> APLNAARPAEERAALLAWVKERLHEEYGDQDPTPRRDPMHELISTILSQQTTHADEEAAYQELRTLGDWDAITLAPTDAVAHAIRRSNYPESKAPRIQETLRRIKAAPGGYDLDFLRDLPVKDALKWLTDLPGVGVKTASLVLLFNYARPVFPVDTHVHRVSTRVGVIPRMGEQAAHRALLALLPPDPPYLYELHINFLSHGRQVCTWTRPKCGKCILRERCDAYALYGDKVPSFSEKPVKGEKPAKG

Endonuclease III (EndoIII) is a ubiquitous bifunctional DNA glycosylase belonging to the helix-hairpin-helix (HhH)-GDP superfamily of DNA glycosylases. It is active for a broad range of oxidized pyrimidine lesions, removing numerous forms of modified thymine and cytosine bases from DNA, such as thymine glycol (Tg), a major stable oxidative modification of thymine, via the Base Excision Repair (BER) pathway. The crystal structures of EndoIIIs from E. coli (EcEndoIII) D. radiodurans (DrEndoIII1 and DrEndoIII3) and G. stearothermophilus (GsEndoIII) revealed that these enzymes comprise two domains divided by a positively charged DNA binding cleft containing the HhH motif and the catalytic residues Asp and Lys. D. radiodurans possesses three genes encoding EndoIII-like enzymes (DrEndoIII1, DrEndoIII2 and DrEndoIII3), while other bacteria typically possess one.

DrEndoIII1 displays a lower activity towards the common substrates and act mostly as a monofunctional DNA glycosylase. Previous comparative structural analysis suggested that amino acid substitutions in two DNA interacting loops (DIL1 and DIL2) and in the FeS cluster loop (a structurally conserved DNA binding motif) could be the origin of the reduced activity of DrEndoIII1. In DrEndoIII1 we substituted Arg61 and Tyr100 in DIL1 and DIL2 with the equivalent residues found in DrEndoIII2 (Glu and Leu). Compared to previous analysis of wild-type DrEndoIII1, which results in full product formation using the same enzyme and substrate concentration, DrEndoIII1 R61Q processed approximately one-third (25 nM) of the substrate compared to the native enzyme. Our results demonstrate that the affinity of the DrEndoIII1 mutants for the substrates (with THF:G mispair and C:G pair) is reduced when compared with the wild-type enzyme. In the case of the R61Q mutant, this probably originates from the substitution of a positively charged residue with a neutral one. The crystal structures were determined and refined to resolutions of 1.38, 1.95 and 1.89 Å for DrEndoIII1 R61Q, DrEndoIII1 Y100L and DrEndoIII3 G250T/N251H, respectively. Additionally, the DrEndoIII1 R61Q and Y100L crystal structures include two magnesium ions, and the DrEndoIII3 G250T/N251H crystal structure has two chloride ions.>WTTRGFVFTRHSQTTAIPSCPEGTVPLYSGFSFLFVQGNQRAHGQDLGTLGSCLQRFTTMPFLFCNVNDVCNFASRNDYSYWLSTPALMPMNMAPITGRALEPYISRCTVCEGPAIAIAVHSQTTDIPPCPHGWISLWKGFSFIMFTSAGSEGTGQALASPGSCLEEFRASPFLECHGRGTCNYYSNSYSFWLASLNPERMFRKPIPSTVKAGELEKIISRCQVCMKKRH[8x]

Basement membranes are extracellular structures of epithelia and endothelia that have collagen IV scaffolds of triple α-chain helical protomers that associate end-to-end, forming networks. At the C-termini, interactions occur between the trimeric NC1 domains of two protomers, forming a hexamer of these domains reinforced by sulfilimine cross-links. Recent studies in one of our laboratories revealed that the NC1 domains function as recognition modules, directing the selection and assembly of α-chains into protomers and networks.

Chloride ions were also present in our α1NC1homo, α3NC1homo and α5NC1homo structures at two different positions in the protomer–protomer interface. Our crystal structures of the α3NC1 and α5NC1 homohexamers provide the first view of the arrangement of the EA and EB regions, which are known critical components of two epitopes that reside in the dissociated α3 and α5 subunits of native α345NC1 hexamers. In the homohexamers these regions are exposed on the surface and are presumably unreactive to antibody binding, as they are in the native α345NC1 hexamers. In Goodpasture’s disease autoantibodies directed to the α3NC1 and α5NC1 domains are generated. Anti-α3NC1 autoantibodies are found in most Goodpasture’s disease patients. The preference of Goodpasture antibodies to recognize the α3NC1 chain could be explained by its sequence composition, although the recent description of Goodpasture’s disease with autoantibodies reactive exclusively to α5NC1 opens the door to additional factors being implicated in pathogenesis. The very recent report of the existence of the α5NC1 homohexamer in vivo gives credence to the view that the canonical α1NC1 and α3NC1 homohexamers presented here may also exist in vivo, particularly given their structural stability, their proper binding of chloride ions for hexamer stabilization and their correct disposition of the residues that mediate the sulfilimine cross-linking bonds that stabilize the hexamer. Solvent-accessibility analysis of residues at the EA and EB epitopes in the α3NC1 and α5NC1 structures, in comparison to the corresponding residues in α1NC1, showed similar exposed surface areas in either monomers or hexamers.>[4x]GAMGRNDNGAIRVYASSTIGNYILPEIIARYRRDFPDLPLEMSVGNSL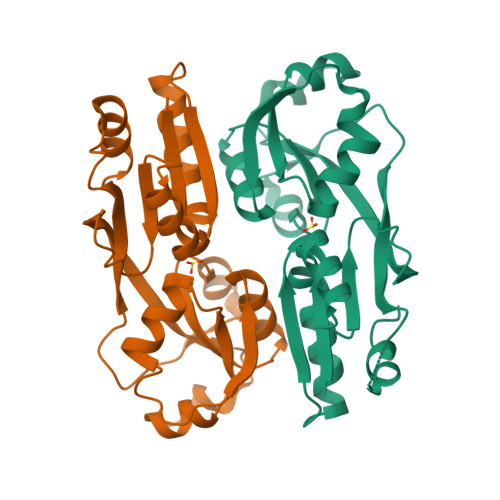DVVQAVCDFRVDIGLIEGPCHMAEIVAQPWLEDELVVFASPASPLLEGEVTLERLAAMPWILREKGSGTREIVDYLLLSHLPQFRLSMELGNSEAIKHAVRHGLGVSCLSRRVIAEQLETGSLVEVKVPLPPLVRTLYRIHHRQKHLSSALARFLRYCEL>[2x]MG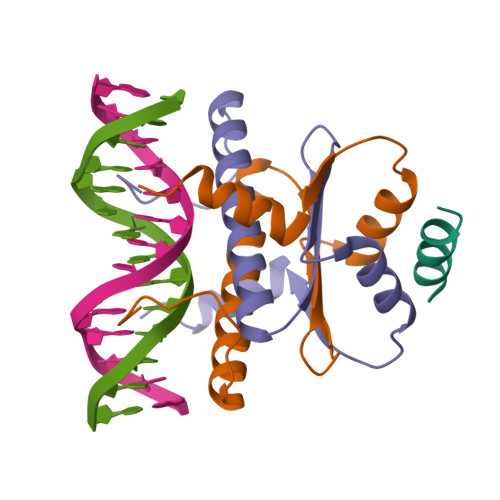RKKIQIQRITDERNRQVTFTKRKFGLMKKAYELSVLCDCEIALIIFNHSNKLFQYASTDMDKVLLKYTEYNEPHESRTNADIIETLRKKGFNG;> GVVKQKLAEVILKKQ>SDGTWQGKQYLKEDGSQAANEWVFDTHYQSWFYIKADANYAENEWLKQGDDYFYLKSGGYMAKSEWVEDKGAFYYLDQDGKMKRNAWVGTSYVGATGAKVIEDWVYDSQYDAWFYIKADGQHAEKEWLQIKGK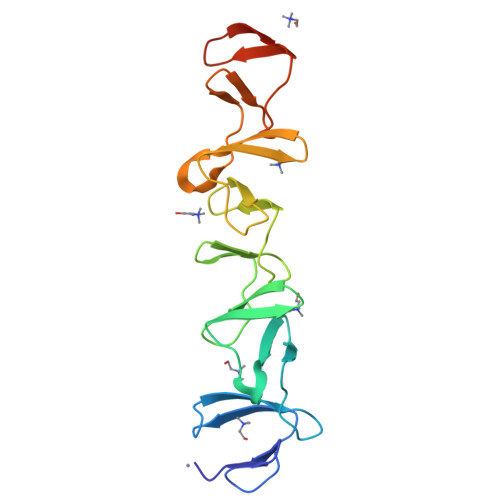DYYFKSGGYLLTSQWINQAYVNASGAKVQQGWLFDKQYQSWFYIKENGNYAD[2x]>GTREKLRKMLDDLLVSVDHSGNIAVLRTPPGGAPFLASFIDRVGMEEVVGTIAGDDTVFVLARDPMTGQEL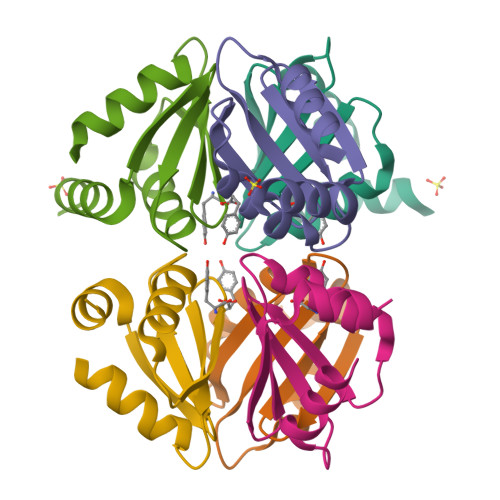GEFLSQRRSGNGGENLYFQGHHHHHH[2x]>MHHHHHHGELKYNCILNIKYEMDRDKLVDSSGYRSRINIGTGVKFSEIDKNQVQLSNLESSKIEVILNNGVIYNSMYENFSTSFWIRIPKYFRNINNEYKIISCMQNNSGWEVSLNFSNMNSKIIWTLQDTEGIKKTVVFQYTQNINISDYINRWIFVTITNNRLSNSKIYINGRLINEESISDLGNIHASNNIMFKLDGCRDPHRYIWIKYFNLFDKELNKKEIKDLYDNQSNSGILKDFWGDYLQYDKPYYMLNLYDPNKYLDVNNVGIRGYMYLKGPRGRIVTTNIYLNSTLYMGTKFIIKKYASGNKDNIVRNNDRVYINVVVKNKEYRLATNASQAGVE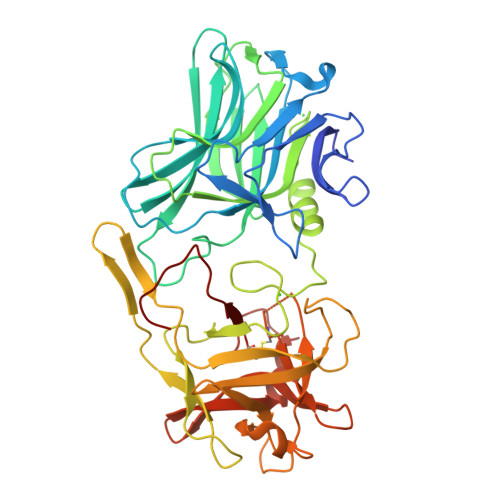KILSAVEIPDVGNLSQVVVMKSENDQGIRNKCKMNLQDNNGNDIGFIGFHQFNNIAKLVASNWYNRQIGKASRTFGCSWEFIPVDDGWGESSL[2x]> MKTPLVTREGYEKLKQELNYLWREERPEVTKKVTWAASLGDRSENADYQYNKKRLREIDRRVRYLTKCMENLKIVDYSPQQEGKVFFGAWVEIENDDGVTHRFRIVGYDEIFGRKDYISIDSPMA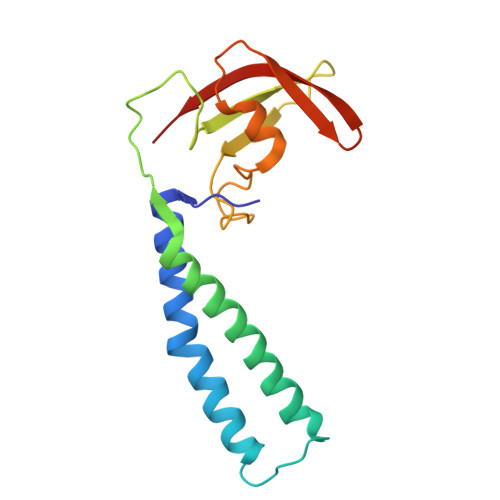RALLKKEVGDLAVVNTPAGEASWYVNAIEYVKP> PVLNLNDPQAVERYEEFMRQSPYGQVTQDLGWAKVKNNWEPVDVYLEDDQGAIIAAMSMLLGDTPTDKKFAYASKGPVMDVTDVDLLDRLVDE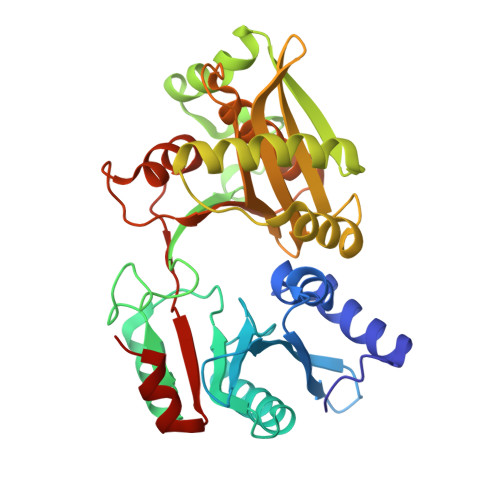AVKALDGRAYVLRFDPEVAYSDEFNTTLQDHGYVTRNRNVADAGMHATIQPRLNMVLDLTKFPDAKTTLDLYPSKTKSKIKRPFRDGVEVHSGNSATELDEFFKTYTTMAERHGITHRPIEYFQRMQAAFDADTMRIFVAEREGKLLSTGIALKYGRKIWYMYAGSMDGNTYYAPYAVQSEMIQWALDTNTDLYDLGGIESESTDDSLYVFKHVFVKDAPREYIGEIDKVLDPEVYAELVKD>MAHHHHHHVDDDDKMITPRFSITQDEEFIFLKIFISNIRFSAVGLEIIIQENMIIFHLSPYYLRLRFPHELIDDERSTAQYDSKDECINVKVAKLNKNEYFEDLDL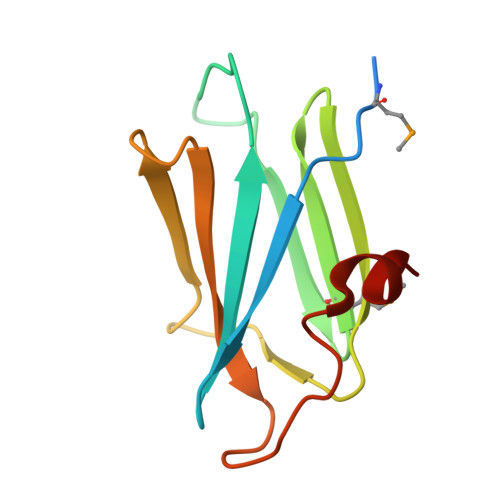PTKLLARQG[6x]> KNNPDPTIYPVLDWNDIKFQDVIGEGNFGQVLKARIKKDGLRMDAAI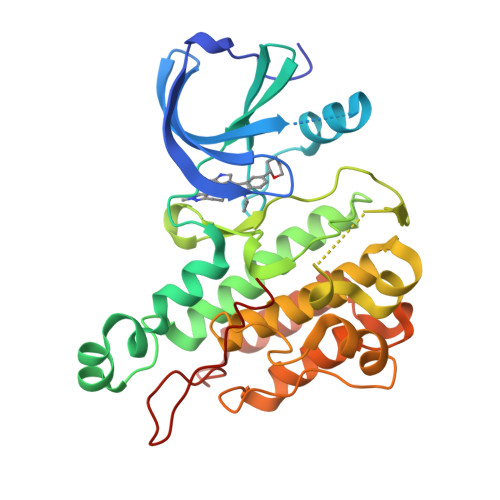KRMKEYASKDDHRDFAGELEVLCKLGHHPNIINLLGACEHRGYLYLAIEYAPHGNLLDFLRKSRVLETDPAFAIANSTASTLSSQQLLHFAADVARGMDYLSQKQFIHRDLAARNILVGENYVAKIADFGLSRGQEVYVKKTMGRLPVRWMAIESLNYSVYTTNSDVWSYGVLLWEIVSLGGTPYCGMTCAELYEKLPQGYRLEKPLNCDDEVYDLMRQCWREKPYERPSFAQILVSLNRMLEERKTYVNTTLYEKFTYAGIDCSAEEAA>[2x]AFIERPEDFLKDKENAIQWEKKEAERVEKNLDTLEKEALELYKKDSEQISNYSQTRQYFYDYQIESNPREKEYKNLRNAISKNKIDKPINVYYFESPEKFAFNKEIRTENQNEISLEKFNELKETIQDKLFKQDGFKDVSLYEPGNGDEKPTPLLIHLKLPKNTGMLPYINSNDVKTLIEQDYSIKIDKIVRIVIEGKQYIKAEASIVNSLDFKDDVSKGDLWGKENYSDWSNKLTPNELADVND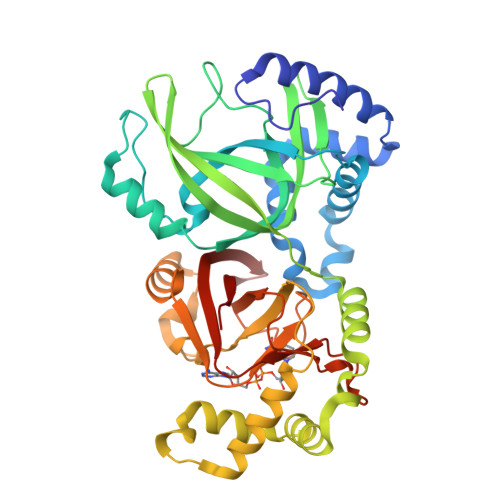YMRGGYTAINNYLISNGPLNNPNPELDSKVNNIENALKLTPIPSNLIVYRRSGPQEFGLTLTSPEYDFNKIENIDAFKEKWEGKVITYPNFISTSIGSVNMSAFAKRKIILRINIPKDSPGAYLSAIPGYAGEYEVLLNHGSKFKINKVDSYKDGTVTKLILDATLIN>SNAMDGEYHSPYGDDDLYTVQPTERSPRDPKAGEDVILNITTWPIENGQDVWVEWTKNGVAQENVTAAYDYNSGNNTYWKADLGKFEKGDEITYTTKGSTNGGTAYESGPFTFYVTDWEYVQDVTSVVDNGDSITLNMTATAGDFSPKLYLSFEDLDTLRMELSPTGKETGHAGKSGYTVEDTAEKVTVTTEDLSIEIQKSPYRMEVHQADGTLLTSEYTTANSLGWLTDGKNVINQYQNNFMTPSDEAFYGFGERYDTINQRGKDVETYVYNEYQDQAQTERTYLAVPFFVSANKYGMYVNSDFHSQFQMASKVEDKYSFVLDNDGDMTNMLDYYVISGKDQNDIVNNYTDITGKTTLLPKWAFGLWMSANEWDRESDVSSALSNAKANDIPATGFVLEQWSDEETYYIWNNATYTAKKNGEAFSYDDFTFNGKWTDPKGMVDSVHDAGMNIVLWQVPVLKDDGTVYEQRDNDEEYMISQGYSADDGTGAPYRVPASQWFGNGILLDFTNKDAVDWWTSQREYLLTEVGIDGFKTDGGEMVWGRDTTFSNGEKGQEMRNRYPTDYVSSYFDFAKSINPEAVSFSRSGTSGAQKSGIYWSGDQTSTFDSFQASLKAGLSASTSGVSYWAWDMAGFTGDYPT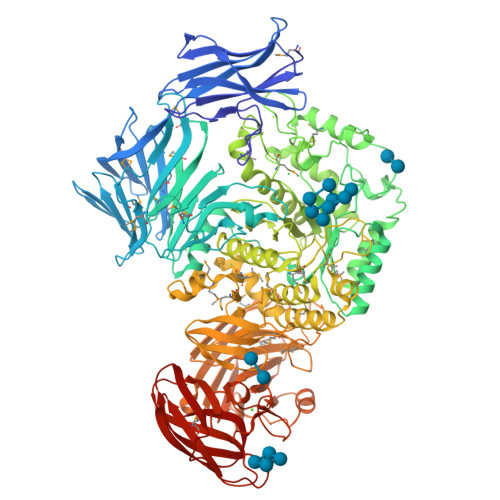AELYKRATAMAAFAPIMQFHSEKSDPSPSEERSPWNAVARTGDETILPTFQKYLYTRMNLLPYIYTAAKDTADNGKSMMRQMAMDYPEDVNARDLDEQYMFGDDLLVAPIVQEGQTEKEVYLPEGEWVDIWNGGVHPGGETISYYADVDTLPVFAKAGAIIPMNMTDGYQLGQNVGNDLKSYDNLTFRVYPSGDSEYSFYDDVNGGEMRDISVSEDFANEKVSVDLPAMADETTMQVFSTEPTSVTIDGADVAKADTLDAFNEATTGYYYDTVQNLTYVKAAAKDAKQAIVLNGVNHAPYEAEFGHLTNVTTASDHAGYTGTGFVAGFDAEKEAVEFDIDAVDGASDYTMEVRYSAGVEDATRTVYINGKKQQITLPKTANWDTWNTVEVPVTLQAGNNQVVFDFEADDTAGINFDHVVIKK[2x]>MSAIKPDMKINLRMEGNVNGHHFVIDGDGTGKPFEGKQSMDLEVKEGGPLPFAFDILTTAFHYGNRVFAEYPDHIQDYFKQSF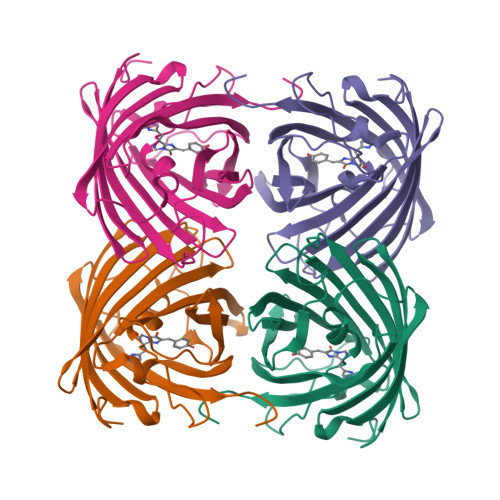PKGYSWERSLTFEDGGICIARNDITMEGDTFYNKVRFHGVNFPANGPVMQKKTLKWEPSTEKMYVRDGVLTGDITMALLLEGNAHYRCDFRTTYKAKEKGVKLPGYHFVDHCIEILSHDKDYNKVKLYEHAVAHSGLPDNARR[4x]> SNAMTIKRKKVSVIGAGFTGATTAFLLAQKELADVV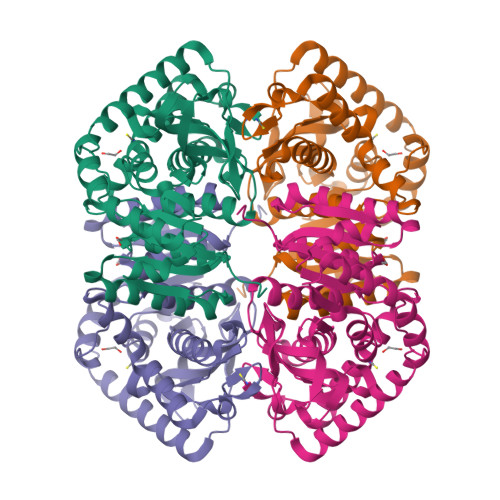LVDIPQLENPTKGKALDMLEASPVQGFDANIIGTSDYADTADSDVVVITAGIARKPGMSRDDLVATNSKIMKSITRDIAKHSPNAIIVVLTNPVDAMTYSVFKEAGFPKERVIGQSGVLDTARFRTFIAQELNLSVKDITGFVLGGHGDDMVPLVRYSYAGGIPLETLIPKERLEAIVERTRKGGGEIVGLLGNGSAYYAPAASLVEMTEAILKDQRRVLPAIAYLEGEYGYSDLYLGVPVILGGNGIEKIIELELLADEKEALDRSVESVRNVMKVLV> MALGPAAMGYDRAITIFSPDGSLYQVDYAFEAVKRGWTTLGVKTKSGVVLLAEKRKATQLLDVDGIEKIFMLDDHVGCTFAGLASDGRILIDYARSQALQHRLIYDEPISIEYLTKVISDVKQAYTQHGGVRPFGVALIVGGIDKGKQPK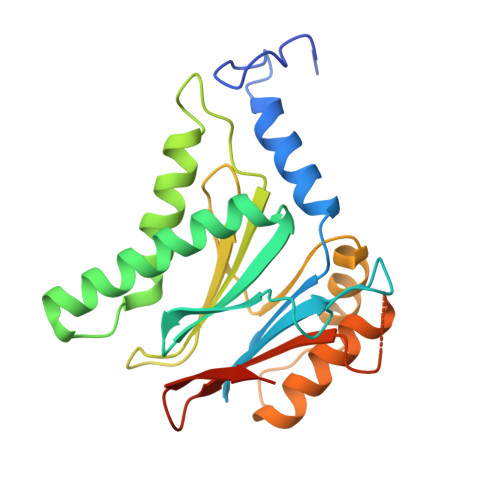LLMTEPSGQFMPYYAVAIGQGGYTATEYLEKNYKEDLDIQSTILLALRALMATLKPGEKLNYSSVEIGYADVDSGTFKKLTTEERSDLLQKI>MGHHHHHHHHHHSSGHIDDDDKHMPEGAALTEKTDIFESGRNGKPNKDGIKSYRIPALLKTDKGTLIAGADERRLHSSDWGDIGMVIRRSEDNGKTWGDRVTITNLRDNPKASDPSIGSPVNIDMVLVQDPETKRIFSIYDMFPEGKGIFGMSSQKEEAYKKIDGKTYQILYREGEKGAYTIRENGTVYTPDGKATDYRVVVDPVKPAYSDKGDLYKGNQLLGNIYFTTNKTSPFRIAKDSYLWMSYSDDDGKTWSAPQDITPMVKADWMKFLGVGPGTGIVLRNGPHKGRILIPVYTTNNVSHLNGSQSSRIIYSDDHGKTWHAGEAVNDNRQVDGQKIHSSTMNNRRAQNTESTVVQLNNGDVKLFMRGLTGDLQVATSKDGGVTWEKDIKRYPQVKDVYVQMSAIHTMHEGKEYI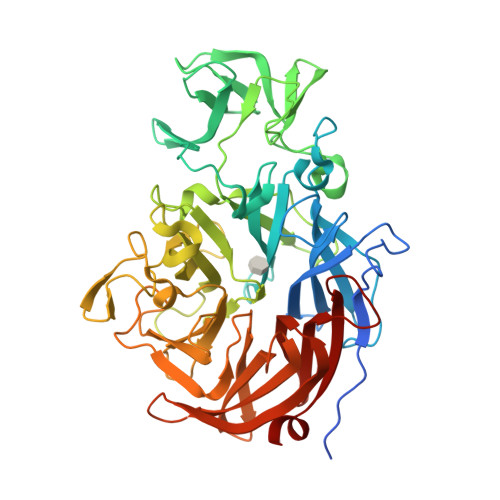ILSNAGGPKRENGMVHLARVEENGELTWLKHNPIQKGEFAYNSLQELGNGEYGILYEHTEKGQNAYTLSFRKFNWDFLSK[2x]> LRAREAKRKATLRMLRESL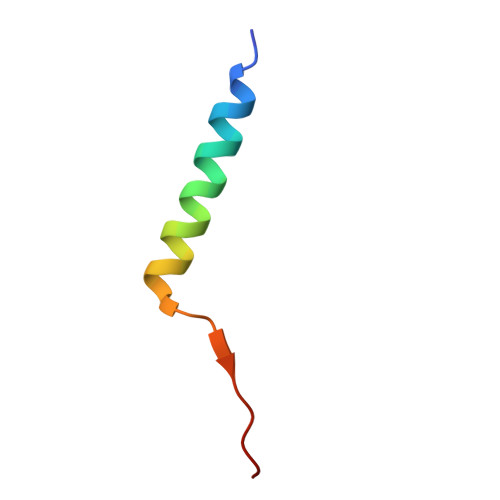ARVGPNVVRLRDD2-{[6-{3-[AMINO(IMINO)METHYL]PHENOXY}-4-(DIISOPROPYLAMINO)-3,5-DIFLUOROPYRIDIN-2-YL]OXY}-5-[(ISOBUTYLAMINO)CARBONYL]BENZOIC ACID | C30 H35 F2 N5 O5 | 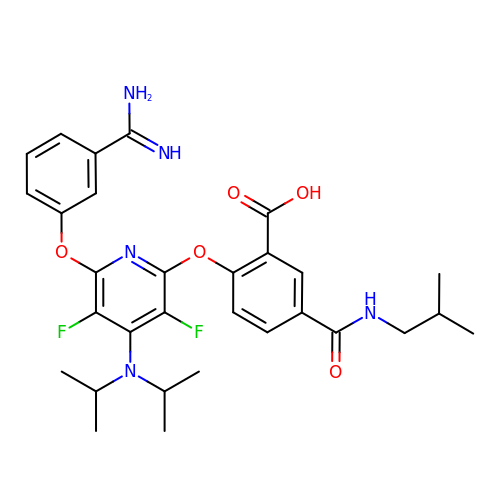JLWMMYZWEHHTFF-UHFFFAOYSA-N>MGTDNTTPAATAETLPYKNPDLPAGERIADLLSRMTLEEKVGQMMQLDARGGDLEDLIVNKHVGSILHTSPEDLSRAAKTVNEKTRLGIPLIIGDDCIHGYSFWPGATIFPSQLGMAVSWDPDKVKAAGRATAEEVSCTGVHWTFSPVLCIARDTRWGRVDETFGEDPMLIGELASAMVKGYQGGAKAGEALPKNAILACAKHFAGYSETQGGRDASEADLSHRKLESWFLPPFERVAKEGCGTFMLGYESIEGVPVTFNKWLLTDKLRGAWKYNGTLITDWDNIGRSVWEQHVKPDYVHAAADAVKAGNDLVMTTPQFYEGAIEAVKTGLLDESLIDDAVSRILALKFRLGLFEDPRLPDAERIKAVIGSAEHQQINLELVRESIALLRNDGALPFAANKVKRIAVVGPLADDAQNQLGDWTGNSGQVSWMPDGQPRDMITTVLDGLTQLTADDCEVVYSRGANVIDLVPDPAGEFYPDGQPRPKIGVSAAVDQALIDEAVANARQSDLIVAVVGDVVQLVGETCSTATLELLGGQNALLDALAAVSRETGKPMVTVLISSKPQVLPASIVGEYGVFAKRVSDPETGTGSILWAPNPGMRGGQAIAEIILGLTNPSGRLPITFPRHAGQLPVYYNQIRGQHGDRYADLTQDPAFAFGEGLSYTTFAYGEPTIVGGASNADGTFAETDTVHAEITLTNTGERAGVEIVQAYIGDIVTSYSWTDRELKAFQRVALEPGETKTVAFEIPVANCTIVDPDANRIVEPGEFELLIGHSSRREDLKRTTFTVALEH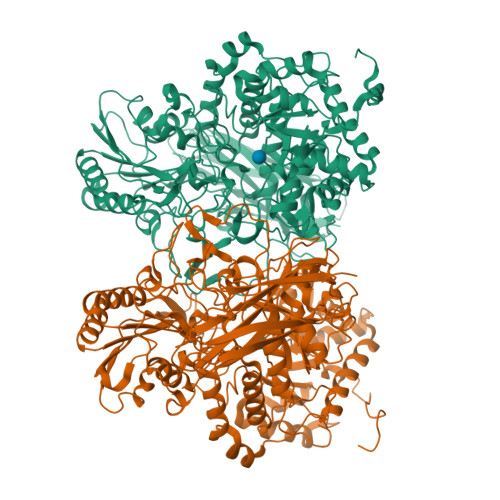HHHHH[2x]Hexameric MCM rings act as the replicative DNA helicase, encircling the leading strand DNA template at the replication fork. Mcm2-7 complexes are loaded to encircle double-stranded DNA (dsDNA) via a ‘gate’ between Mcm2 and Mcm5 to yield a double hexamer that does not unwind DNA. During helicase activation, the Dbf4-dependent Cdc7 kinase (DDK) and cyclin-dependent kinases (CDKs) drive recruitment of Cdc45 and the GINS complex. These factors stimulate the Mcm2-7 ATPase and helicase and with Mcm2-7 form the CMG complex (Cdc45-Mcm2-7-GINS), the active replicative helicase. Following activation, two Mcm2-7 helicases encircle single-stranded DNA (ssDNA) and translocate independently, 3ʹ→5ʹ, on the leading strand DNA template with the ATPase domain leading.

We tested the DNA unwinding activity of PfMCMAAA to compare with that of the Sso-PfMCM chimera to explore interdomain communication. We found PfMCMAAA had a negligible unwinding activity. The inactivity of PfMCMAAA could result from attributes identified in the PfMCMAAA double-octamer crystal structure (see ‘Materials and methods’). Specifically, the non-hexameric ring architecture or the alternative topology for the helix-2-insert region, both of which we consider artifacts of the N-terminal truncation, could fully explain the lack of unwinding by this domain. Thus, although SsoMCMN does enhance the unwinding activity of PfMCMAAA, this could simply be due to enforcing a hexameric architecture or by disallowing the unusual h2i topology in favor of the canonical topology.

>[16x]SPEEEQIIKELAKRKDIVDAIVDSIAPAIYGYKEVKKGIALALFGGVSRKLPDGTRLRGDIHVLLVGDPGVAKSQILRYVANLAPRAIYTSXXXXXXXXXXXXXXXXXXXXXXXXXXXXXXXXXGGYALIDELDKMSDRDRSVIHEALEQQTISISKAGITATLNARTTVIAAANPKQGRFNRMKNPFEQIDLPPTLLSRFDLIFVLIDEPDDKIDSEVARHILRVRRGESEVVAPKIPHEILRKYIAYARKNIHPVISEEAMEEIEKYYVRMRKSVKKTKGEEEGIPPIPITARQLEALIRLSEAHARMRLSPIVTREDAREAIKLMEYTLKQIAMD>MVSANGDLHLPISNEQCMPENNGSLGFEAPTPRQILRVTLNLKYLIDKVVPIVYDPNDIVCDHSEILSPKVVKLAYEACGGNPKDKANKRKYQSVIIFSLLKVCEWYSILATMEVHNAKLYETRNLASQQLCKLLIEREETRDLQFLFMQLLLRRYVINENDEDQEPLNALELATDMHCTTVIGSSGFQRCLKWIWRGWIVQNGLDPTTFIKDDSLAEVSLISHFNPVRLKAPVYQNYLQMIFSFLFLGLYTLVVNGKDSERVQSFDLLESIFYVFNTGFILDELTKLYYIGYAHLSFWNLFNDTTYLIITFAMGFRAMSVTPLNAKYSSEDWDKISYRVLSCAAPFVWSRLLLYLESQRFIGIMLVILKHMMKESIVFFFLLFLIMIGFTQGFLGLDSADGKRDITGPILGNLTITVLGLGSFDVFEEFAPPYAAILYYGYYFIVSVILLNILIALYSTAYQKVIDNADDEYMALMSQKTLRYIRAPDEDVYVSPLNLIEVFMTPIFRILPPKRAKDLSYTVMTIVYSPFLLLISVKETREARRIKYNRMKRLNDDANEYDTPWDLTDGYLDDDDGLFSDNRNSGMRATQLKNSRSLKLQRTAEQEDVHFKVPKKWYKNVKKCSPSFEQYDNDDTEDDAGEDKDEVKELTKKVENLTAVITDLLEKLDIKDKKE[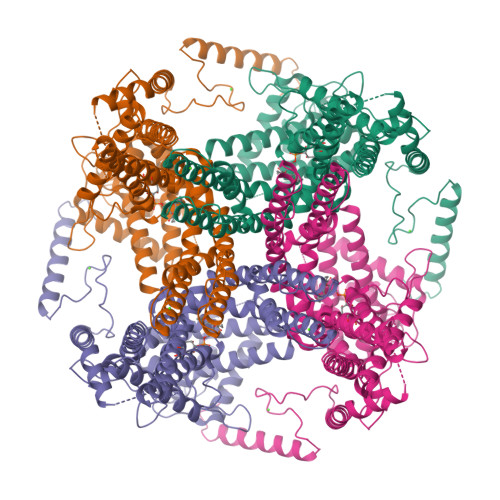4x]> MSTYDEIEIEDMTFEPENQMFTYPCPCGDRFQIYLDDMFEGEKVAVCPSCSLMIDVVHHHHHH;> MSCVYAFGSNGQRQLGLGHDEDMDTPQRSVPGDDGAIVRKIACGGNHSVMLTNDGNLVGCGDNRRGELDSAQALRQVHDWRPVEVPAPVVDVACGWDTTVIVDADGRVWQRGGGCYEFTQQHVPLNSNDERIAVYGCFQNFVVVQGTRVYGWGSNTKCQLQEPKSRSLKEPVLVYDTGSVAVDYVAMGKDFMVIVDEGGRIVHASGRLPTGFELKQQQKRHNLVVLCMWTSIHLWNARLNTVESFGRGTHSQLFPQERLDFPIVGVATGSE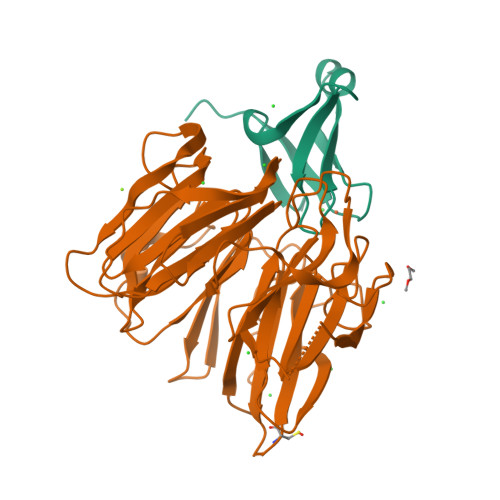HGILTTANQEGKSHCYNVYCWGWGEHGNCGPQKGSQPGLQLVGQYSGKPRVFGGCATTWIVL(3R)-3-methyl-4-{6-[1-(S-methylsulfonimidoyl)cyclopropyl]-2-(naphthalen-1-yl)pyrimidin-4-yl}morpholine | C23 H26 N4 O2 S | 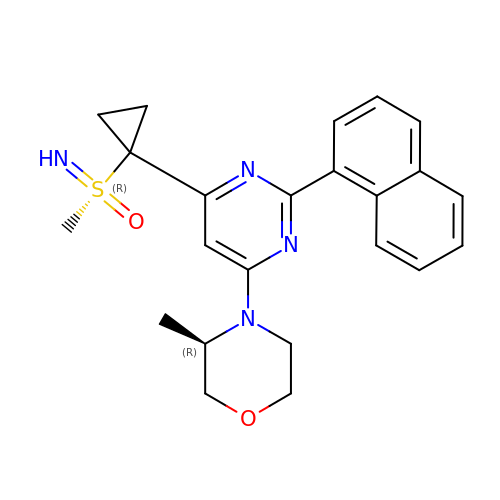GOXNOBRASUTVOC-XHDOVSQSSA-N> MSD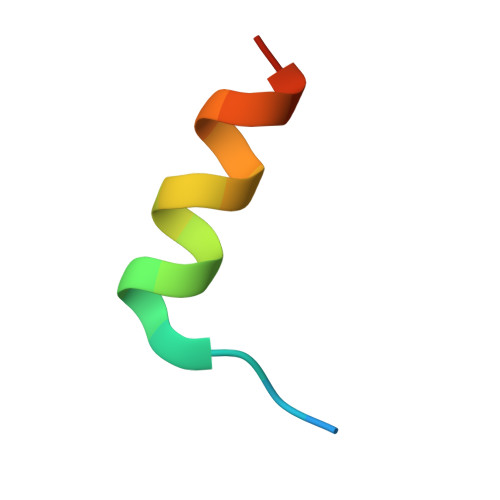VLSQEEINQLIEALMKG> TMAASQTSQTVASHVPFADLCSTLERIQKSKGRAEKIRHFREFLDSWRKFHDALHKNHKDVTDSFYPAMRLILPQLERERMAYGIKETMLAKLYIELLNLPRDGKDALKLLNYRTPTGTHGDAGDFAMIAYFVLKPRCLQKGSLTIQQVNDLLDSIASNNSAKRKDLIKKSLLQLITQSSALEQKWLIRMIIKDLKLGVSQQTIFSVFHNDAAELHNVTTDLEKVCRQLHDPSVGLSDISITLFSAFKPMLAAIADIEHIEKDMKHQSFYIETKLDGERMQMHKDGDVYKYFSRNGYNYTDQFGASPTEGSLTPFIHNAFKADIQICILDGEMMAYNPNTQTFMQKGTKFDIKRMVEDSDLQTCYCVFDVLMVNNKKLGHETLRKRYEILSSIFTPIPGRIEIVQKTQAHTKNEVIDALNEAIDKREEGIMVKQPLSIYKPDKRGEGWLKIKPEYVSGLMDELDILIVGGYWGKGSRGGMMSHFLCAVAEKPPPGEKPSVFHTLSRVGSGCTMKELYDLGLKLAKYWKPFHRKAPPSSILCGTEKPEVYIEPCNSVIVQIKAAEIVPSDMYKTGCTLRFPRIEKIRDDKEWHECMTLDDLEQLRGKASGK;> DVPQWEVFFKR

DNA ligase IV (LigIV), one of three DNA ligases in higher eukaryotes, plays a central role in the repair of DNA double-strand breaks (DSBs) during nonhomologous end joining (NHEJ). Human DNA ligases have a conserved catalytic region consisting of a DNA-binding domain (DBD), a nucleotidyltransferase domain (NTD), and an OB-fold domain (OBD) (Tomkinson et al., 2006). A covalent AMP-lysine intermediate is formed with the catalytic lysine (K273) in motif I of LigIV (step 1) before the AMP is transferred to the 5′ phosphate of the DNA nick (step 2). Artemis is activated by the autophosphorylation of DNA-PKcs (Goodarzi et al., 2006). It has recently been found that Artemis (residues 485–495) also interacts with LigIV (Malu et al., 2012).

Here, we report the crystal structure at 2.4 Å resolution of the catalytic region of LigIV (residues 1–609) in complex with an Artemis peptide. The crystallographic structure of Artemis485–495 in complex with mercury-labeled LigIV1–609, in which nine mercury atoms are coordinated by cysteines and methionines, was determined at 2.4 Å resolution using the multiwavelength anomalous dispersion (MAD) method. The structures proved to be very similar except for the conformation of the loop between β11 and β12, which is distorted by the binding of thiomersal in the mercury derivative (data not shown). In the derivative crystals of the LigIV1–609/Artemis485–495 complex, the poor density for adenosine is consistent with partial adenylation as observed by DNA ligation assay. Although density for the αPO4 is evident, it is likely that AMP has low occupancy. The density of β and γ phosphates is absent in the derivative crystals, probably because ATP diffuses from the binding site while the crystals are soaking in thiomersal solution, as observed by others (Håkansson et al., 1997; Pascal et al., 2006). Artemis485–495 interacts with α1 and α2 of LigIV to form a three-helix bundle, burying 436 Å2 of the surfaces of LigIV1–609 and Artemis485–495. α1 has a kink produced by the proline P15, which is conserved in higher eukaryotic organisms. W489 of Artemis (italic font for the residues of Artemis), which is an important conserved residue for LigIV interaction (Malu et al., 2012), makes a hydrogen bond from its Nε to the side chain of D18 of LigIV. It also makes van der Waals contacts with the conserved V14 in a hydrophobic pocket of LigIV, the conformation of which is constrained by I145 in α7 of LigIV. The interaction of the side chain of W489 of Artemis in the hydrophobic pocket appears to be stabilized by further interactions of F492 of Artemis with F49 of LigIV and F493 of Artemis with F42 of LigIV, consistent with the earlier report that W489, F492, and F493 mutations to alanines disrupt the interaction between Artemis and LigIV (Malu et al., 2012).> RWAPIPCSMLENSLGPFPLFLQQVQSDTAQNYTIYYSIRGPGVDQEPRNLFYVERDTGNLYCTRPVDREQYESFEIIAFATTPDGYTPELPLPLIIKIEDENDNYPIFTEETYTFTIFENCRVGTTVGQVCATDKDEPDTMHTRLKYSIIGQVPPSPTLFSMHPTTGVITTTSSQLDRELIDKYQLKIKVQDMDGQYFGLQTTSTCI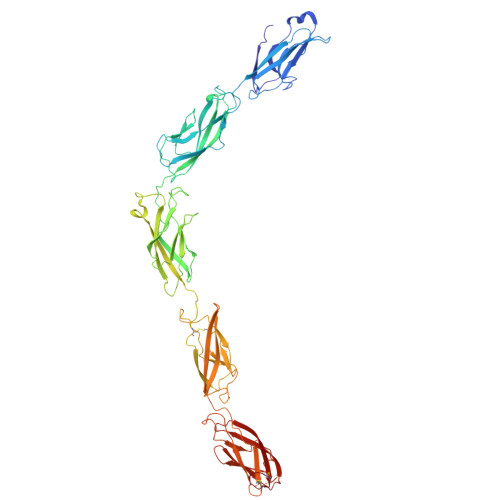INIDDVNDHLPTFTRTSYVTSVEENTVDVEILRVTVEDKDLVNTANWRANYTILKGNENGNFKIVTDAKTNEGVLCVVKPLNYEEKQQMILQIGVVNEAPFSREASPRSAMSTATVTVNVEDQDEGPECNPPIQTVRMKENAEVGTTSNGYKAYDPETRSSSGIRYKKLTDPTGWVTIDENTGSIKVFRSLDREAETIKNGIYNITVLASDQGGRTCTGTLGIILQDVNDNSPFIPKKTVIICKPTMSSAEIVAVDPDEPIHGPPFDFSLESSTSEVQRMWRLKAINDTAARLSYQNDPPFGSYVVPITVRDRLGMSSVTSLDVTLCDCITENDCTH1-(5-deoxy-beta-L-xylofuranosyl)pyrimidine-2,4(1H,3H)-dione | C9 H12 N2 O5 | 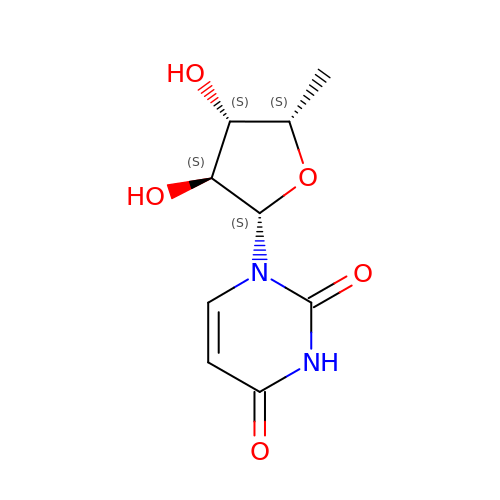WUBAOANSQGKRHF-UCVXFZOQSA-N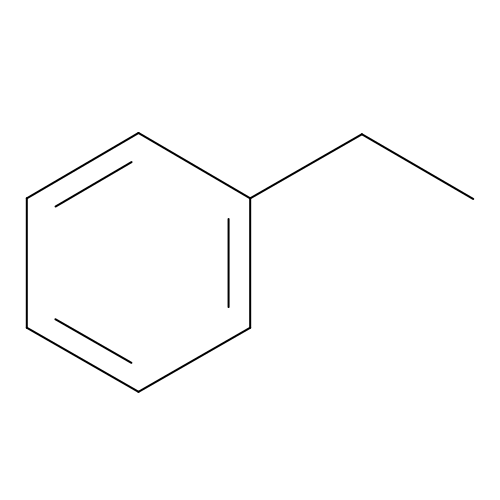PHENYLETHANE | C8 H10 | YNQLUTRBYVCPMQ-UHFFFAOYSA-N>[3x]GPHMSTEKAPAALGPYSQAIKANNLVFLSGVLGLIPETGKFVSESVEDQTEQVLKNMGEILKASGADYSSVVKTTIMLADLADFKTV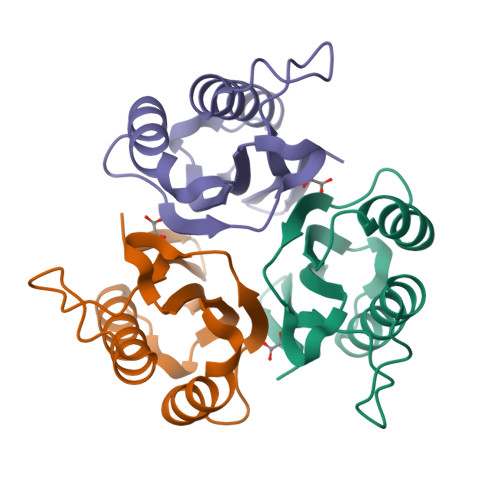NEIYAKYFPAPSPARSTYQVAALPLNAKIEIECIATL>ASNFDCCLGYTDRILHPKFIVGFTRQLANEGCDINAIIFHTKKKLSVCAN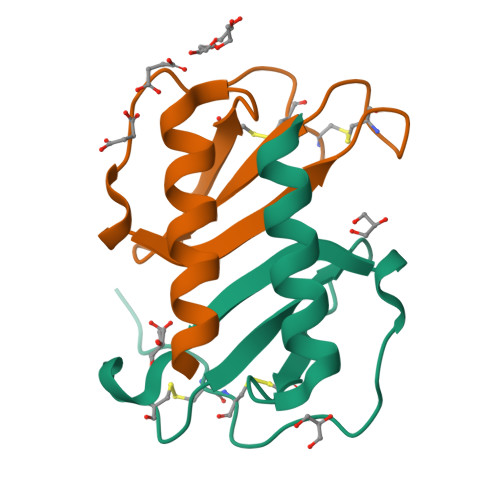PKQTWVKYIVRLLSKKVKNM[5x]> MENNGYKIILIGS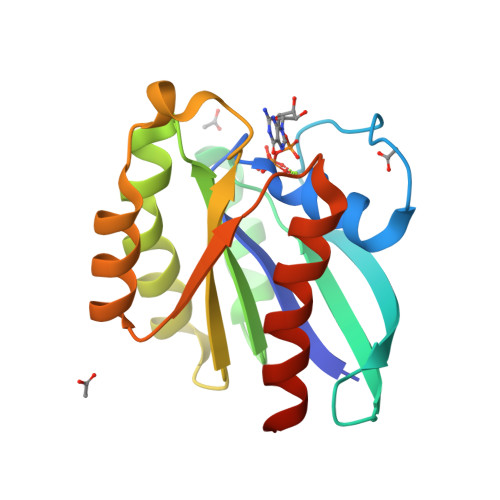SGVGKSSIVHQFLFNRKISNVSPTIGAAFASKQVIAKNGKTLKLNIWDTAGLERFRSITKMYYTNSLGCLVVFDVTDRESFDDVYYWINDLRINCHTTYYILVVANKIDIDKNNWRVSENEIKKFCRDNDCDYVFASSFESDTVNNLFGKMIDKMSEIKINPD> MAFKRHIDRLPIIPADAKKHNVTCHFCIVGCGYHAYTWPINKQGGTDPQNNIFGVDLSEQQQAESDAWYSPSMYNVVKQDGRDVHVVIKPDHECVVNSGLGSVRGARMAETSFSEARNTQQQRLTDPLVWRYGQMQPTSWDDALDLVARVTAKIVKEKGEDALIVSAFDHGGAGGGYENTWGTGKLYFEAMKVKNIRIHNRPAYNSEVHGTRDMGVGELNNCYEDAELADTIVAVGTNALETQTNYFLNHWIPNLRGESLGKKKELMPEEPHEAGRIIIVDPRRTVTVNACEQTAGADNVLHLAINSGTDLALFNALFTYIADKGWVDRDFIDKSTLREGTARPPLYPARGVSEANPGHLSSFEDAVEGCRMSIEEAAEITGLDAAQIIKAAEWIGMPKEGGKRRRVMFGYEKGLIWGNDNYRTNGALVNLALATGNIGRPGGGVVRLGGHQEGYVRPSDAHVGRPAAYVDQLLIGGQGGVHHIWGCDHYKTTLNAHEFKRVYKKRTDMVKDAMSAAPYGDREAMVNAIVDAINQGGLFAVNVDIIPTKIGEACHVILPAATSGEMNLTSMNGERRMRLTERYMDPPGQSMPDCLIAARLANTMERVLTEMGDVGYAAQFKGFDWQTEEDAFMDGYNKNAHGGEFVTYERLSAMGTNGFQEPATGFTDGKIEGTQRLYTDGVFSTDDGKARFMDAPWRGLQAPGKQQQKDSHKYLINNGRANVVWQSAYLDQENDFVMDRFPYPFIEMNPEDMAEAGLKEGDLV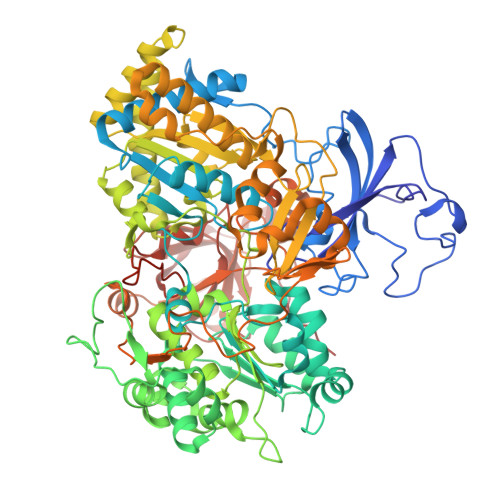EIYNDAGATQAMAYPTPTARRGETFMLFGFPTGVQGNVTSAGTNELIIPNYKQTWGNIRKISDAPRNVAHLSFKSKEYQSA Processivity factors, or sliding clamps, such as the prokaryotic β-clamp and eukaryotic and archaeal proliferating cell nuclear antigen (PCNA), show a high degree of structural conservation despite limited sequence identity. These ring–shaped proteins topologically encircle DNA providing a sliding platform for the majority of DNA polymerases and many DNA-interacting proteins. Most typically these partners bind to the processivity factor via a conserved motif (β-clamp: QL[S/D]LF and PCNA: Qxx[I/L/M]xxF[F/Y]) at their extreme N- or C-terminus, although internal motifs are not unknown. Pol V is a heterotrimer consisting of the catalytic UmuC subunit and a homodimer of UmuD’ and was originally identified as being central to damage-induced mutagenesis.

The structure of the E. coli β-clamp was solved in complex with a fluorophore-labelled synthetic UmuC β-binding peptide to 2.5 Å resolution. The asymmetric unit contains a single β-clamp dimer with a peptide bound to each monomer. The 12-mer peptide consisted of Dylight649-C-QGVAQLNLFDD363, with a cysteine included to permit linkage of the fluorophore to the peptide. Residues 356AQLNLF361 were modelled for chain D and 357QLNLF361 for chain C, comprising the core β-binding motif of the UmuC peptide, with the remaining residues presumably disordered. The OE1 group forms a hydrogen bond with a conserved solvent molecule, with the NE2 group forming two hydrogen bonds with the main chain carbonyls of Met-362 and Pro-363 on the clamp. The density for peptide Asn-359 is well-defined, due to a hydrogen bond formed between its OD1 group and the NH2 group of Arg-152 on the clamp surface. Peptide Leu-360 is located within the hydrophobic pocket on the clamp surface defined by residues Val-247, Leu-177, Val-360, Pro-242, Met-362, with the main chain nitrogen forming a hydrogen bond with the carbonyl group of Gly-174. Remarkably, and in contrast to the other peptide-clamp complexes, peptide Phe-361 does not penetrate the hydrophobic pocket of the clamp and is solvent exposed. The principle interaction appears to be hydrophobic in nature, with the hydrophobic portion of the clamp Arg-246 side chain. We suggest that greater reliance is placed upon the UmuC Asn-359 to clamp Arg-152 interaction, since no intimate interaction exists between UmuC Phe-361 and the clamp, with Phe-361 involvement limited instead to interaction with the hydrophobic portion of the side chain of clamp Arg-246.

>HHHHHHMKFTVEREHLLKPLQQVSGPLGGRPTLPILGNLLLQVADGTLSLTGTDLEMEMVARVALVQPHEPGATTVPARKFFDICRGLPEGAEIAVQLEGERMLVRSGRSRFSLSTLPAADFPNLDDWQSEVEFTLPQATMKRLIEATQFSMAHQDVRYYLNGMLFETEGEELRTVATDGHRLAVCSMPIGQSLPSHSVIVPRKGVIELMRMLDGGDNPLRVQIGSNNIRAHVGDFIFTSKLVDGRFPDYRRVLPKNPDKHLEAGCDLLKQAFARAAILSNEKFRGVRLYVSENQLKITANNPEQEEAEEILDVTYSGAEMEIGFNVSYVLDVLNALKCENVRMMLTDSVSSVQIEDAASQSAAYVVMPMRL[2x];>[2x]CQGVAQLNLFDD>GSAAFNAWRNTPKSLINLKEIEPQLATDPDSAFFWSGRTEGVGGPDVAEAIAKSRGGVTLESTIKDKNIKMPEWDFDNPQSIKAWEDV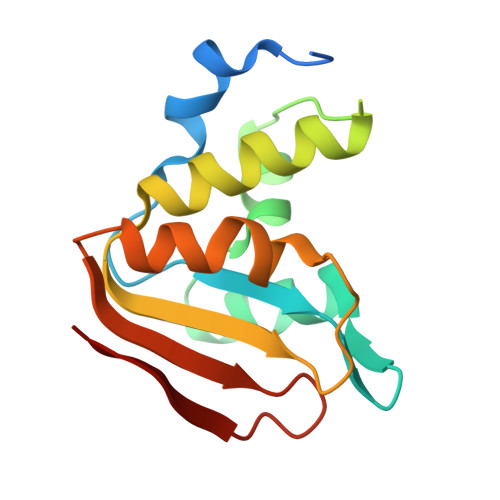SASYAKQVSGEVRAVVGQSLREGNIWENVELPRLMGNDNVTKITTIDPLSQTEKVIFVRDN[2x]> SDALKVRWPDFNQEAYVGGTMVRSGQDPYARNKFNQVESDKLRMDRAIPDTRHDQCQRKQWRVDLPATSVVITFHNEARSALLRTVVSVLKKSPPHLIKEIILVDDYSNDPEDGALLGKIEKVRVLRNDRREGLMRSRVRGADAAQAKVLTFLDSHCECNEHWLEPLLERVAEDRTRVVSPIIDVINMDNFQYVGASADLKGGFDWNLVFKWDYMTPEQRRSRQGNPVAPIKTPMIAGGLFVMDKFYFEELGKYDMMMDVWGGENLEISFR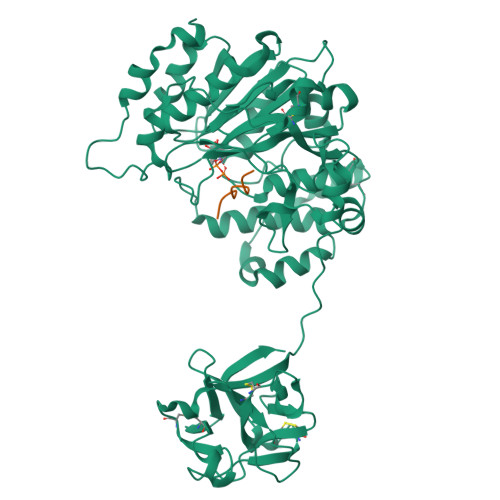VWQCGGSLEIIPCSRVGHVFRKQHPYTFPGGSGTVFARNTRRAAEVWMDEYKNFYYAAVPSARNVPYGNIQSRLELRKKLSCKPFKWYLENVYPELRVPDHQDIAFGALQQGTNCLDTLGHFADGVVGVYECHNAGGNQEWALTKEKSVKHMDLCLTVVDRAPGSLIKLQGCRENDSRQKWEQIEGNSKLRHVGSNLCLDSRTAKSGGLSVEVCGPALSQQWKFTLNLQQ;> PTTDSTTPAPTTK> GPLGSENVPEKDLHGRLFINRIFHISADRMFELLFTSSRFMQKFASSRNIIDVVSTPWTAELGGDQLRTMTYTIVLNSPLTGKCTAATEKQTLYKESREARFYLVDSEVLTHDVPYHDYFYTVNRYCIIRSSKQKCRLRVSTDLKYRK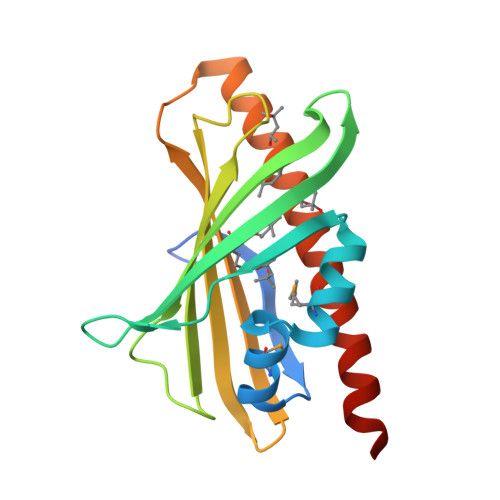QPWGLVKSLIEKNSWSSLEDYFKQLESDLLIEESVLNQAIEDPG>GAMPVTTPTKMATLTTKQMWQTIKDYFGDGFVTGSAPISYNVHTCDMQLQPDSGIHAASDGIHYGVQISEDSMPLFSIMGDTAAPPCTCHRVDEIVKHIDEFLERAPEALPDDGAITSGKPCDTNPDQVSLYAMRDSLSWWVHWGGNLRPEHYWKQIYIGFAAIPDDVQISPREFLDGTYRYLGHTWDDCLSGLEEEGVSPDEIEFANMCMWRQMLTQWLEKADPELLPLLKGKISLMLQYRVLTANTLGCLALFMNATADPKDGPIHYADSSYEMEIASVAQCVTLDMAKEAMGILQGERTEVVAGD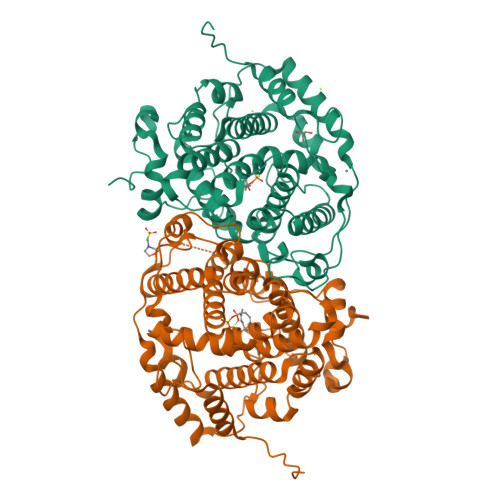RAQRKRELRWIYVRCMQILESQPHAHMLRRYGSAGLHYVPMMDRYLERVSGHTRFPIRDGAARILERFINRAELPKESEDINPNGRSLKVSAKMNGNGQLHHEVNGNAKLHLEAERPDVTTAVG[2x]5-(7-fluoranyl-3,3-dimethyl-2-oxidanylidene-1H-indol-5-yl)-4-methyl-1H-pyrazole-3-carbonitrile | C15 H13 F N4 O | 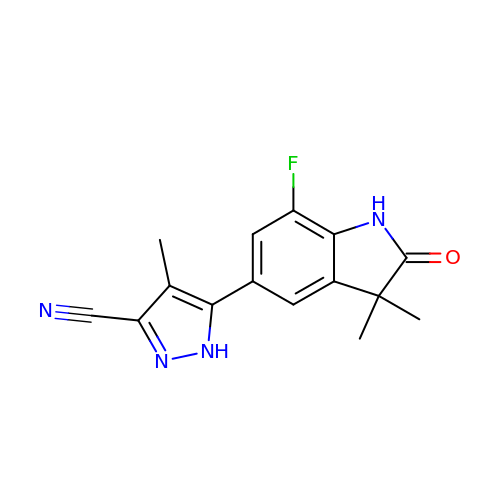OQCSCPAZLQNXQT-UHFFFAOYSA-N>[4x]DSELISENMHMKLYMEGTVNDHHFKCTSEGEGKPYEGTQTMKIKVVEGGPLPFAFDIL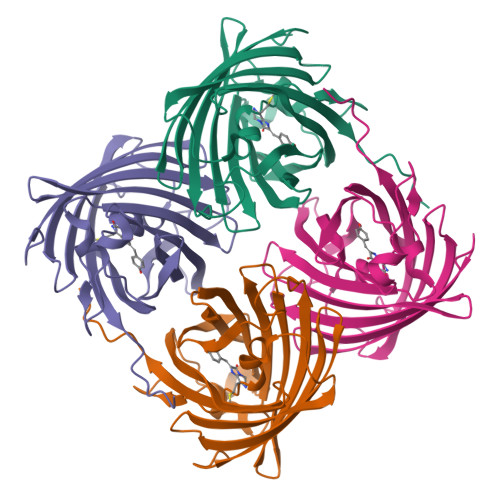ATSFMYGSKTFINHTQGIPDFFKQSFPEGFTWERITTYEDGGVLTATQDTSLQNGCLIYNVKINGVNFPSNGPVMQKKTLGWEASTEMLYPADSGLRGHSQMALKLVGGGYLHCSLKTTYRSKKPAKNLKMPGFYFVDRKLERIKEADKETYVEQHEMAVARYCDLPSKLGHS>REFMAVTANNSQLLTWWHNTGEINTQTPVADGNVRQSGLYSVKVQTTPASSSLYYDSFVYLAIP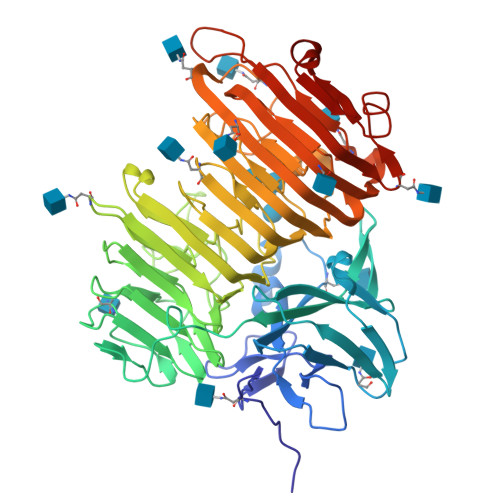GNGMSDQLQYTQGYNQTQAWTSFLYSHDATVKISRNGSSANSNVVIRPTSLNFPVRYDNQSVYITVPYSPTGYRFSVEFDDDLISLAPSGARQPENALLIFASPFENSSTKPQPGSPNSIAPAPGRVLGLNTTSASTVVFNPGVYYFTGHDHMVLSSSVTWVYFAPGAYVKGAVEFLSTASEVKASGHGVLSGEQYVWYADPDEGYQKASGANNNGLRMWRGTLGNSSQTFVLNGVTVSAPPFNSMDWSGNSLDLITCRVDDYKQVGAFYGQTDGLEMYPGTILQDVFYHTDDDGLKMYYSNVTARNIVMWKESVAPVVEFGWTPRNTENVLFDNVDVIHQAYANAGNNPGIFGAVNNYLYAPDGLSSNHSTGNSNMTVRNITWSNFRAEGSSSALFRINPIQNLDNISIKNVSIESFEPLSINTTESWMPVWYDLNNGKQITVTDFSIEGFTVGNTTITASNAASVGRIDGVDPAYAGSVHYID[2x]> MEINVSKLRTDLPQVGVQPY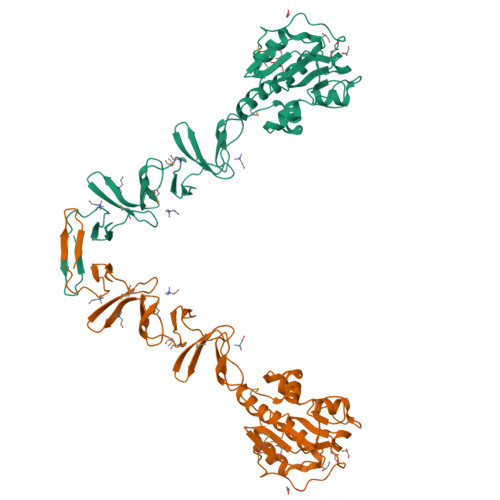RQVHAHSTGNPHSTVQNEADYHWRKDPELGFFSHIVGNGCIMQVGPVDNGAWDVGGGWNAETYAAVELIESHSTKEEFMTDYRLYIELLRNLADEAGLPKTLDTGSLAGIKTHEYCTNNQPNNHSDHVDPYPYLAKWGISREQFKHDIENGLTIETGWQKNDTGYWYVHSDGSYPKDKFEKINGTWYYFDSSGYMLADRWRKHTDGNWYWFDNSGEMATGWKKIADKWYYFNEEGAMKTGWVKYKDTWYYLDAKEGAMVSNAFIQSADGTGWYYLKPDGTLADKPEFTVEPDGLITVK>[2x]GPVSVAN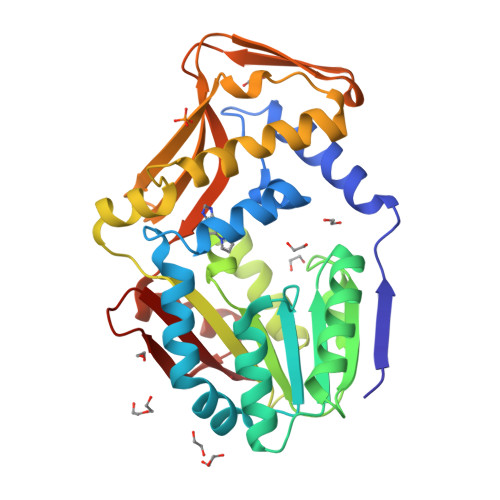HLGEDAGHLALRRDVYSGLQKTPKSLPPKWFYDTVGSELFDQITRLPEYYPTRAEAEILRARSAEVASACRADTLVELGSGTSEKTRMLLDALRHRGSLRRFVPFDVDASVLSATATAIQREYSGVEINAVCGDFEEHLTEIPRGGRRLFVFLGSTIGNLTPGPRAQFLTALAGVMRPGDSLLLGTDLVKDAARLVRAYDDPGGVTAQFNRNVLAVINRELEADFDVDAFQHVARWNSAEERIEMWLRADGRQRVRVGALDLTVDFDAGEEMLTEVSCKFRPQAVGAELAAAGLHRIRWWTDEAGDFGLSLAAK(2R)-6,8-dichloro-7-(2-methylpropoxy)-2-(trifluoromethyl)-2H-chromene-3-carboxylic acid | C15 H13 Cl2 F3 O4 | 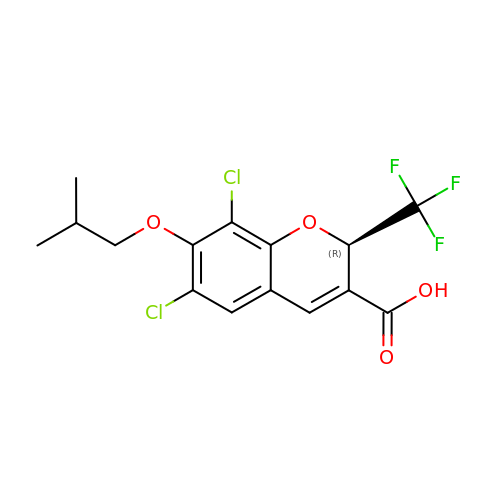FQKMILFVTQADHR-CYBMUJFWSA-N>HHHHHHSSGLVPRGSHMASMSKVGINGFGRIGRLVLRRLLEVKSNIDVVAINDLTSPKILAYLLKHDSNYGPFPWSVDFTEDSLIVDGKSIAVYAEKEAKNIPWKAKGAEIIVECTGFYTSAEKSQAHLDAGAKKVLISAPAGEMKTIVYNVNDDTLDGNDTIVSVASCTTNCLAPMAKALHDSFGIEVGTMTTIAAYTGTQSLVDGPRGKDLRASRAAAENIIPHTTGAAKAIGLVIPELSGKLKGHAQRVPVKTGSVTELVSILGKKVTAEEVNNALKQATT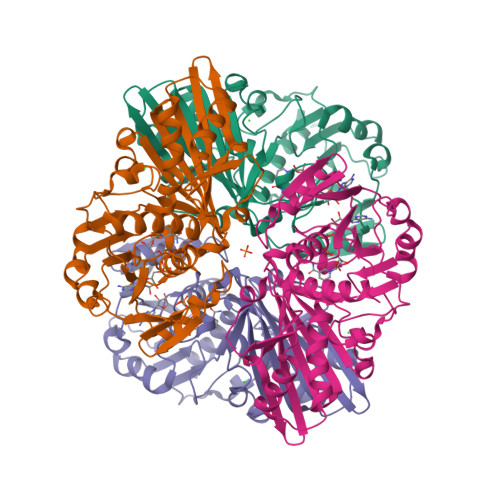NNESFGYTDEEIVSSDIIGSHFGSVFDATQTEITAVGDLQLVKTVAWYDNEYGFVTQLIRTLEKFAKL[4x]> AYDRAITVFSPDGRLFQVE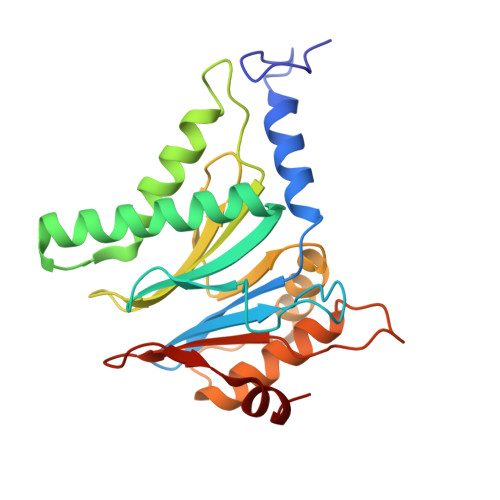YAREAVKKGSTALGMKFANGVLLISDKKVRSRLIEQNSIEKIQLIDDYVAAVTSGLVADARVLVDFARISAQQEKVTYGSLVNIENLVKRVADQMQQYTQYGGVRPYGVSLIFAGIDQIGPRLFDCDPAGTINEYKATAIGSGKDAVVSFLEREYKENLPEKEAVTLGIKALKSSLEEGEELKAPEIASITVGNKYRIYDQEEVKKFL> QGGGRMRKKLYNDFAWECLRRNPQYISDWELFMKNTLTNGGGIPDDSELIQSELDLNAEKKWGVMKYIDPYNSDPTNVFWSLKLSNRSVRVKLSNTGNVKGGYTWGDMSNLPGVKHQRLLMHDNTLCVKIFSQNGYFQLFIESADALKDXXXXXXXXXXXXXXXXXXXXXXXXX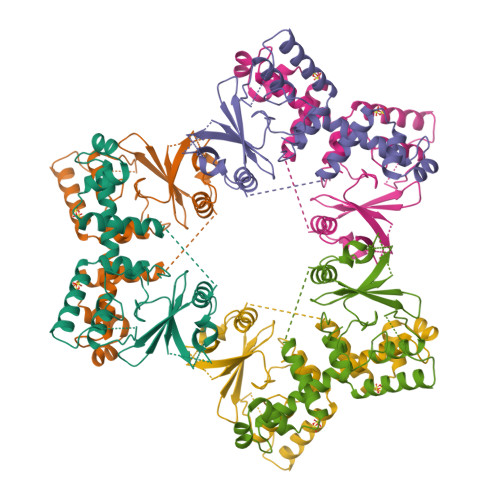XIVNHKIEVECKEEQYLGLLKTIDDRKQGFSHRDIASEIFGKELVKNEWSADSWVRAKIRYRIKKANALINYGYLNFL In bacteria, uridine 1915 of the 23S rRNA undergoes two steps of post-transcriptional modification—pseudouridylation, followed by N3-methylation—that convert it to 3-methylpseudouridine (m3Ψ). RlmH acts on the assembled 70S ribosome. RlmH consists of five parallel β-strands (β2-β1-β4-β3-β5) sandwiched between two layers of α-helices: α2 and α4 on the solvent side, and α1, α5 and α3 on the dimerization interface. Our data suggest that E. coli RlmH functions as a dimer, with the SAM binding pocket of one monomer and the C-terminal residues of its counterpart forming a composite active site.

The crystal structures of E. coli RlmH bound to the cofactor SAM or to the inhibitor sinefungin contain two dimers of RlmH in an asymmetric unit, with two cofactors bound to each RlmH dimer. Each of the two cofactors (SAM and sinefungin) binds to RlmH in a bent conformation in which the amino-acid moiety of the cofactor folds toward the adenine base. Three bights (U-shaped, curved sections) of the overhand knot define the SAM-binding pocket. Bight 1 (loop β3–α3) and bight 3 (loop β5–α5) shape the hydrophobic core, which hosts the adenine moiety of SAM. Interactions with residues L72, I74, L122, L127, V132 and the backbone carbonyls of L125 and S123 secure the adenine base. The ribose of SAM interacts mainly with bight 2 (β4–α4). The reactive methyl group in SAM is sandwiched between the backbone atoms of bights 2 and 3. The methyl group faces the C-terminus of the partner RlmH monomer, where the RNA substrate likely binds. Comparing the structure of SAM-bound and ligand-free enzyme shows that cofactor binding rearranges the C-terminal loop into a 310-helix in each subunit. Our SAM-bound structure reveals that SAM binding shifts the C-terminus of RlmH by as much as 14 Å, rearranging it into a 310 helix (close-up).

>[4x]MHHHHHHVKLQLVAVGTKMPDWVQTGFTEYLRRFPKDMPFELIEIPAGKRGKNADIKRILDKEGEQMLAAAGKNRIVTLDIPGKPWDTPQLAAELERWKLDGRDVSLLIGGPEGLSPACKAAAEQSWSLSALTLPHPLVRVLVAESLYRAWSITTNHPYHRE>MTQELGNANFENFIGATEGFSEIAYQFTSHILTLGYAVMLAGLLYFILTIKNVDK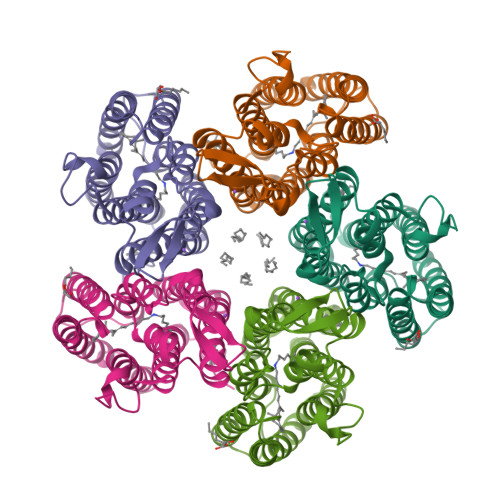KFQMSNILSAVVMVSAFLLLYAQAQNWTSSFTFNEEVGRYFLDPSGDLFNNGYRYLNWLIDVPMLLFQILFVVSLTTSKFSSVRNQFWFSGAMMIITGYIGQFYEVSNLTAFLVWGAISSAFFFHILWVMKKVINEGKEGISPAGQKILSNIWILFLISWTLYPGAYLMPYLTGVDGFLYSEDGVMARQLVYTIADVSSKVIYGVLLGNLAITLSKNKELVEANSLEHHHHHH[5x]>GFDYDVVVVGGGFAGATAARECGLQGYRTLLLEARSRLGGRTFTSRFAGQEIEFGGAWVHWLQPHVWAEMQRYGLGVVEDPLTNLDKTLIMYNDGSVESISPDEFGKNIRIAFEKLCHDAWEVFPRPHEPMFTERARELDKSSVLDRIKTLGLSRLQQAQINSYMALYAGETTDKFGLPGVLKLFACGGWNYDAFMDTETHYRIQGGTIGLINAMLTDSGAEVRMSVPVTAVEQVNGGVKIKTDDDEIITAGVVVMTVPLNTYKHIGFTPALSKGKQRFIKEGQLSKGAKLYVHVKQNLGRVFAFADEQQPLNWVQTHDYSDELGTILSITIARKETIDVNDRDAVTREVQKMFPGVEVLGTAAYDWTADPFSLGAWAAYGVGQLSRLKDLQAAEGRILFAGAETSNGWHANIDGAVESGLRAGREVKQLLS[2x]

Nicotine oxidoreductase (NicA2) is a flavin-dependent enzyme that catalyzes the degradation of nicotine into the non-psychoactive metabolite N-methylmyosmine (NMM). NicA2 acts by degrading nicotine in the bloodstream before it reaches the brain. Clinical use of NicA2 is limited by its poor catalytic activity in the absence of its natural electron acceptor CycN. The higher in vivo activity of NicA2 is due to the presence of a cytochrome c, termed CycN, that acts as an alternative electron acceptor to O29.

Inspection of the solvent-accessible surface area in the crystal structure of wild-type NicA2 revealed several interconnected cavities that extend from the si-side of the FAD isoalloxazine moiety to the surface. One such tunnel is in a region that is rich with the mutations that we discovered that improve the oxidase activity of NicA2. We previously determined that NMM formed due to nicotine oxidation remains bound to wild-type NicA2 when it is oxidized by its natural electron acceptor CycN9. By contrast, the NMM-bound structures of v321 and wild-type NicA2 are very similar with an overall root mean squared deviation of <0.5 Å and no obvious difference that would explain our observed change in activity with O2. The addition of NMM did not cause any notable chemical shift perturbation in wild-type NicA2, although the peak narrowed, suggesting that ligand binding may restrict conformational fluctuations in the tunnel. The major populations of both wild-type NicA2 and NicA2 v321 appear less accessible to solvent when bound by NMM than when ligand free. We have succeeded in isolating variants of NicA2 that are much more capable of reacting with O2 than the wild-type enzyme (koxO2 of 28 M−1 s−1 when bound by NMM).> HQYLLPEAKAQDSDKICVVINLDETLVHSSFKPVNNADFIIPVEIDGVVHQVYVLKRPHVDEFLQRMGELFECVLFTASLAKYADPVAD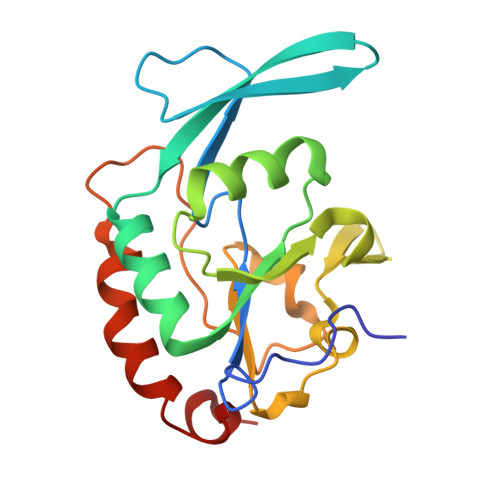LLDKWGAFRARLFRESCVFHRGNYVKDLSRLGRDLRRVLILDNSPASYVFHPDNAVPVASWFDNMSDTELHDLLPFFEQLSRVDDVYSVLRQ> MAHHHHHHMAARTDDPRLLSLFSAQREEDADIVIIGFPYDEGCVRNGGRAGAKKGPAAFRFFLQRLGSVNNLELNVDASHLKLYDAG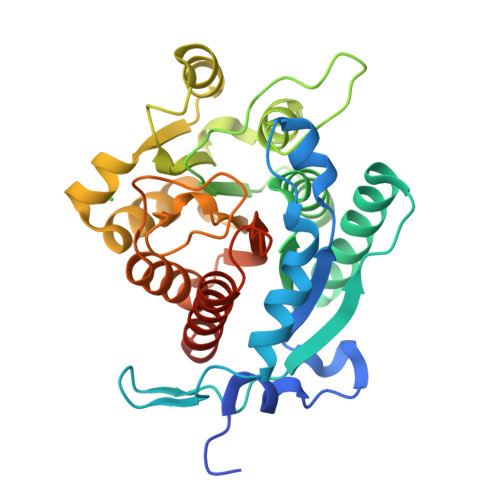DITASTLEEAHEKLESKVFTVLARGAFPFVIGGGNDQSAPNGRAMLRAFPGDVGVINVDSHLDVRPPLQDGRVHSGTPFRQLLEESSFSGKRFVEFACQGSQCGALHAQYVRDHQGHLMWLSEVRKKGAVAALEDAFGLTGKNTFFSFDVDSLKSSDMPGVSCPAAVGLSAQEAFDMCFLAGKTPTVMMMDMSELNPLVEEYRSPRVAVYMFYHFVLGFATRPKPKAEN> MECPFQIQVCISDRFFAFPHNLVEPQSDVGNKLIENLIVYVPTDDDRLYIDKKQFPKFNSVLVYRHEHDVNIDSRSPKKTASATIVYWNPLVPITEIGAGETRVFSVLLTNNLFYCNTMIVHHENPKCPIEFTYPETDMQSACSALLKNRNGQSVPPPIKSNLRPIACEIPLSHFKELVESNDFLLCFNLETSTMVKILSLKRIFCIFQYRKQPARYVINLPHEEIDNLYNKLNWERTRRLMKGDVPSNCATVNRSSLKYIKQAQSLLGIPDYSQTVVDFVKMFQKIIFPYQLVPNVIIKLNNFDQMVSSAPNKAEPYKKIRLFCKNDSIAISSSGIVPINMPDFSPPNT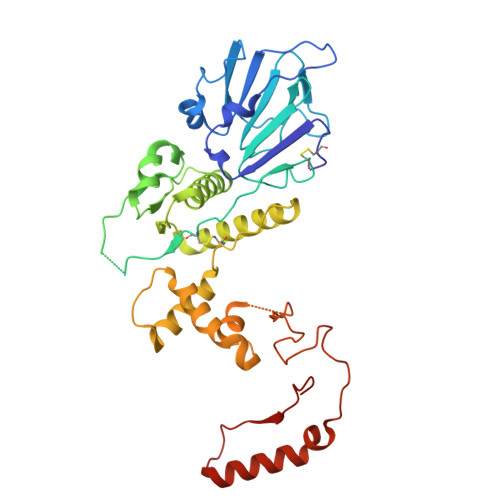FDYSDYANRTNINFVTQRVLTDGGFSSGITVTPVKYNYYL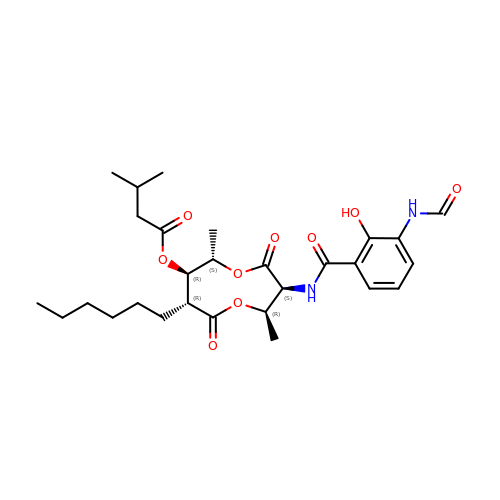[(2R,3S,6S,7R,8R)-3-[(3-formamido-2-oxidanyl-phenyl)carbonylamino]-8-hexyl-2,6-dimethyl-4,9-bis(oxidanylidene)-1,5-dioxonan-7-yl] 3-methylbutanoate | C28 H40 N2 O9 | UIFFUZWRFRDZJC-SBOOETFBSA-N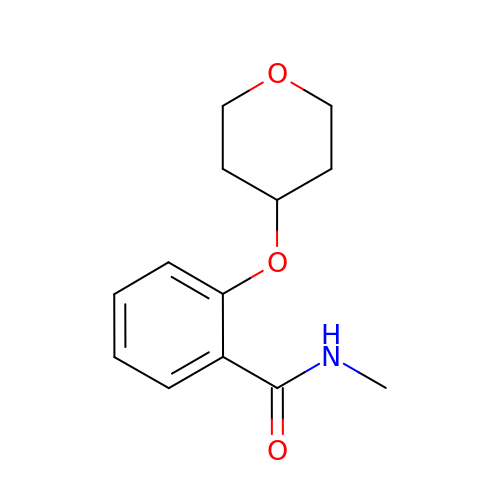N-methyl-2-(tetrahydro-2H-pyran-4-yloxy)benzamide | C13 H17 N O3 | WZBIMVSWUWZIHN-UHFFFAOYSA-N>[4x]MGMWASLDALWEMPAEKRIFGAVLLFSWTVYLWETFLAQRQRRIYKTTTHVPPELGQIMDSETFEKSRLYQLDKSTFSFWSGLYSETEGTLILLFGGIPYLWRLSGRFCGYAGFGPEYEITQSLVFLLLATLFSALAGLPWSLYNT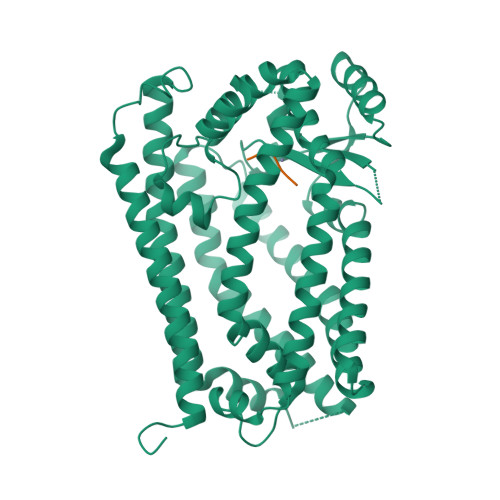FVIEEKHGFNQQTLGFFMKDAIKKFVVTQCILLPVSSLLLYIIKIGGDYFFIYAWLFTLVVSLVLVTIYADYIAPLFDKFTPLPEGKLKEEIEVMAKSIDFPLTKVYVVEGSKRSSHSNAYFYGFFKNKRIVLFDTLLEEYSVLNKDIQEDSGMEPRNEEEGNSEEIKAKVKNKKQGCKNEEVLAVLGHALGHWKLGHTVKNIIISQMNSFLCFFLFAVLIGRKELFAAFGFYDSQPTLIGLLIIFQFIFSPYNEVLSFCLTVLSRRFEFQADAFAKKLGKAKDLYSALIKLNKDNLGFPVSDWLFSMWHYSHPPLLERLQALKTMKQHAENLYFQ;>CSIM[4x]> XGFAFFA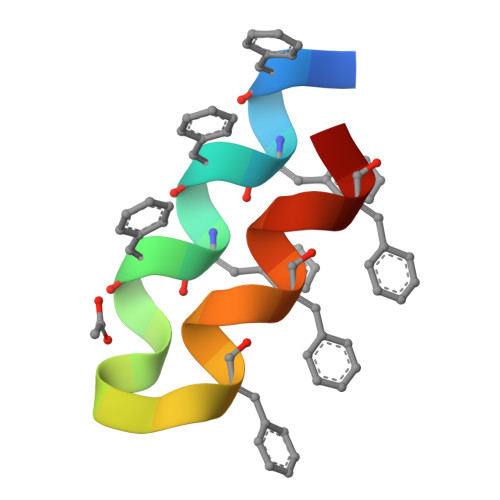FFAGGGGFALFALFAX>[4x]MRKIVVAAIAVSLTTVSITASASADPSKDSKAQVSAAEAGITGTWYNQLGSTFIVTAGADGALTGTYESAVGNAESRYVLTGRYDSAPATD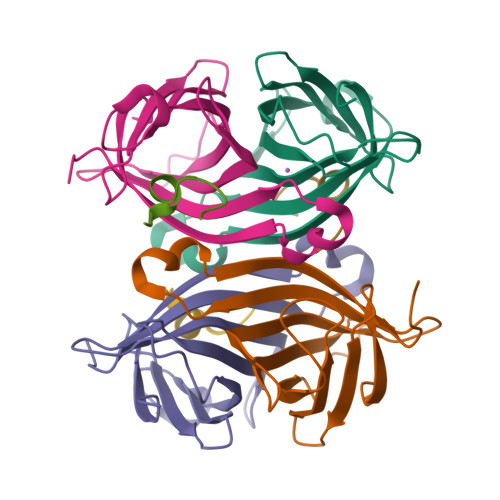GSGTALGWTVAWKNNYRNAHSATTWSGQYVGGAEARINTQWLLTSGTTEANAWKSTLVGHDTFTKVKPSAASIDAAKKAGVNNGNPLDAVQQ;>RDPAPAWAHGGGX[3x]>[2x]MTDRFTRLLGIQQPIIQAPMLGVSTPALAAAVSNAG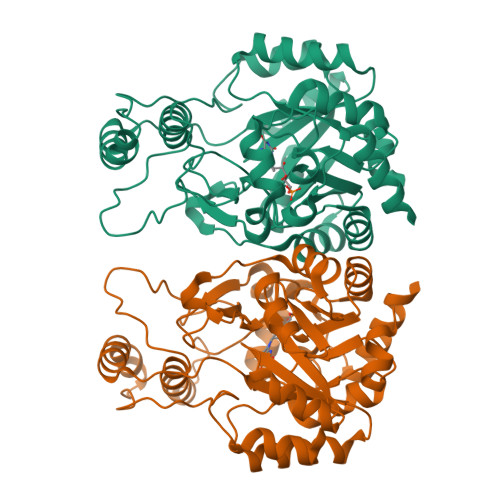GLGSIAITGSAAEKGRALIREVRGLTDKPFNVNLFCHRPGQADPARERAWLDYLKPLFAEFGAEPPVRLKNIYLSFLEDPTLLPMLLEERPAAVSFHFGAPPRDQVRALQAVGIRVLVCATTPEEAALVEAAGADAVVAQGIEAGGHRGVFEPERGDAAIGTLALVRLLAARGSLPVVAAGGIMDGRGIRAALELGASAVQMGTAFVLCPESSANAAYREALKGPRAARTALTVTMSGRSARGLPNRMFFDAAAPGVPPLPDYPFVYDATKALQTAALARGNHDFAAQWAGQGAALARELPAAELLRTLVEELRGHHHHHH>[3x]MDKLISNNKLKLSVVLLGGLCSLAYYHLKNKFHLSQFCFSKKWFSEFSIMWPGQAFSLKIKKILYETKSKYQNVLVFESTTYGKVLVLDGVIQLTEKDEFAYHEMMTHVPMTVSKEPKNVLVVG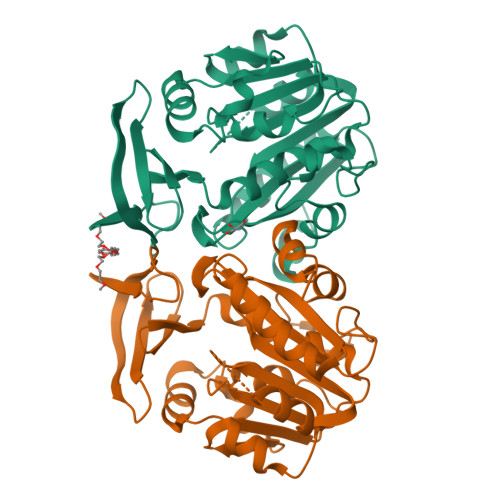GGDGGIIRELCKYKSVENIDICEIDETVIEVSKIYFKNISCGYEDKRVNVFIEDASKFLENVTNTYDVIIVDSSDPIGPAETLFNQNFYEKIYNALKPNGYCVAQCESLWIHVGTIKNMIGYAKKLFKKVEYANISIPTYPCGCIGILCCSKTDTGLTKPNKKLESKEFADLKYYNYENHSAAFKLPAFLLKEIENI The 1-Deoxy-d-xylulose 5-phosphate reductoisomerase (DXR, IspC, EC 1.1.1.267), the second and rate-limiting enzyme in the MEP pathway, catalyzes the isomerization and the reduction of 1-Deoxy-d-xylulose 5-phosphate (DXP) into MEP. The catalysis occurs with dependency of a metallic dication (Mg2+) and NADPH as cofactors. TgDXR is composed of three domains: an N-terminal NADPH-binding domain, a connective domain and a C-terminal α-helical domain. These are arranged in a V shape, where the N-terminal and C-terminal domains form the two arms and the central domain lies at the vertex.

In this study, we present the first crystal structure of T. gondii DXR (TgDXR) in a tertiary complex with the inhibitor fosmidomycin and the cofactor NADPH in dimeric conformation at 2.5 Å resolution revealing the inhibitor binding mode. The asymmetric unit contains one homodimer. NADPH is bound to the Rossmann fold by interactions typically observed, while the pyrophosphate moiety interacts with the consensus sequence GGGNGA, establishing further interactions with the co-substrate NADPH which is bound at the identical position as found in other DXR proteins. The binding of the adenine and pentose phosphate moieties of NADPH is identical to that observed in the structure of the E. coli DXR, in contrast, the nicotinamide ring of NADPH is ordered in this fosmidomycin complex. Within the solvent-shielded cavity that is formed upon closure of the ‘lid’ residues 281–285 the inhibitor backbone lies parallel to the β-indole of Trp283 at a distance of ∼4 Å. The hydroxamic acid moiety of the inhibitor binds to the side-chain of Glu231. The sidechain of Glu231 itself is stabilized and positioned via interaction with Lys299. Fosmidomycin further interacts with the sidechains of Asn298 and His280. The sidechain of Glu302 also points towards the fosmidomycin, however the distance is roughly 4 Å indicating a very weak interaction or maybe this interaction is water mediated which cannot be conclusively modelled at this resolution. Not surprisingly, also the binding site for fosmidomycin at TgDXR consists of the same amino acids as seen in the structure of the EcDXR, indicating that the domain of TgDXR is similar to the EcDXR domain. The distance of the hydroxymate region of fosmidomycin to NADPH is 4.4 Å, which is too large for conversion (indicated by the yellow line in Figure 4C).

>[2x]MGHHHHHHHHHHSSGHIEGRHMSTRVKRLVVLGSTGSIGKSTLEIAREFPDIFQIVGLAAGGSNLALLAEQVAAFRPQYVYLGDSSKVAELQERLNDHERSAAFPRPRLLLGDEGLAELACVPNYDILVSAIVGFKGVLPTLKALEAGKDVALANKEALVAAGPVFRCLLSTRGLLYGDQERQDRHERSHRSGDQEGDREEDTDGDRREECDKRRAKAGQKCGLLLPVDSEHSAIFQALQGVPASCYPPRKLLLTASGGPFRGRTRDELEQVTLESALKHPKWSMGAKITIDSATLMNKGLEVIEAHFAFGCPYSSIEVLVHPQAVIHSAVELRDGATLAQLGLPDMKLPIAYALTWPHRLAAPWSAGVDLTREGNLTFEKPDLNTFGCLGLAYEAGERGGVAPACLNAANEVAVERFRNKEIGFVDIEDTVRHVMALQERERDNFSDVSLQDVFDADHWARTAARAFKPRK> MAKHLFTSESVSEGHPDKIADQISDAVLDAILEQDPKARVACETYVKTGMVLVGGEITTSAWVDIEKITRNTVREIGYVHSDMGFDANSCAVLSAIGQQSPDINQGVDRADPLEQGAGDQGLMFGYATNETDVLMPAPITYAHRLVQRQAEVRKNGTLPWLRPDAKSQVTFQYDDGKIVGIDAVVLSTQHSEEIDQKSLQEAVMEEIIKPILPAEWLTSATKFFINPTGRFVIGGPMGDCGLTGRKIIVDTYGGMARHGGGAFSGKDPSKVDRSAAYAARYVAKNIVAAGLADRCEIQVSYAIGVAEPTSIMVETFGTEKVPSEQLTLLVREFFDLRPYGLIQMLDL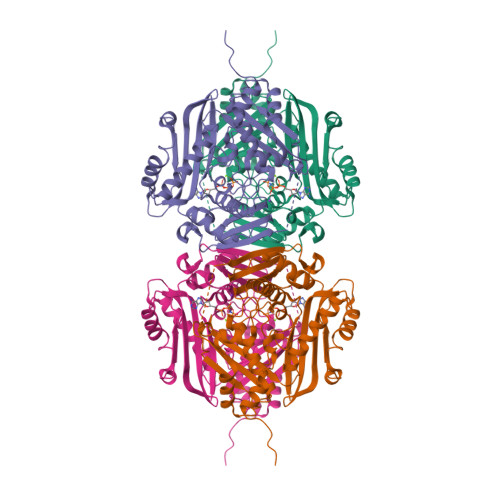LHPIYKETAAYGHFGREHFPWEKTDKAQLLRDAAGLKHHHHHH Protonation of key histidine residues has been long implicated in the acid-mediated cellular action of the diphtheria toxin translocation (T-) domain, responsible for the delivery of the catalytic domain into the cell. The function of the T-domain is to translocate the catalytic domain across the lipid bilayer in response to the acidification of the endosome. Remarkably, such a complex task is performed by this small 180-residue protein without the help of any additional translocation machinery. Formation of the membrane-competent W+-state occurs in solution upon acidification of the environment to pH below 6 and is accompanied by structural destabilization and partial unfolding of the T-domain.

In order to further analyze the putative pH-dependent structuring of the TH2-TH3 region, we crystallized a full-length form of diphtheria toxin (DT) harboring the H223Q/H257Q mutations. Notably, two crystal forms were obtained from crystallization solutions at pH 5.5 and 4.5. The first crystal form (DT-DM-A) was isomorphous with the aforementioned WT structures, whereas the other form (DT-DM-B) belonged to another crystal form. Not surprisingly, the mutant structures also form domain-swapped dimers and are similar to the WT structures. Interestingly, the TH2 helices in the mutant structures are well ordered in a similar manner as observed for the WT pH 7.0 structure and could be modeled on the electron density maps. Interestingly, the Q223/Q257 sidechain conformations are distinctly different from the H223/H257 residues in the WT structures. Moreover, the acid-induced destabilization of the T-domain’s short helix TH2, previously reported for the WT, is no longer observed with the DM. The latter is overall consistent with the spectroscopic evidence presented above in Figure 2 for the lack of efficient conversion of the membrane-competent state in the mutant. The replacement of H223 and H257 with non-titratable Q residues suppresses the ability of the T-domain to form a membrane-competent state and disrupt the bilayer yet has little effect on the protonation of the other four histidines.

>MGADDVVDSSKSFVMENFSSYHGTKPGYVDSIQKGIQKPKSGTQGNYDDDWEGFYSTDNKYDAAGYSVDNENPLSGKAGGVVKVTYPGLTKVLALKVDNAETIKKELGLSLTEPLMEQVGTEEFIKRFGDGASRVVLSLPFAEGSSSVKYINNWEQAKALSVELEINFETRGKRGQDAMYEYMAQACAGNRVRRSVGSSLSCINLDWDVIRDKTKTKIESLKEQGPIKNKMSESPNKTVSEEKAKQYLEEFHQTALEQPELSELKTVTGTNPVFAGANYAAWAVNVAQVIDSETADNLEKTTAALSILPGIGSVMGIADGAVHHNTEEIVAQSIALSSLMVAQAIPLVGELVDIGFAAYNFVESIINLFQVVHNSYNRPAYSPGHKTQPFLHDGYAVSWNTVEDSIIRTGFQGESGHDIKITAENTPLPIAGVLLPTIPGKLDVNKSKTHISVNGRKIRMRCRAIDGDVTFCRPKSPVYVGNGVHANLHVAFHRSSSEKIHSNEISSDSIGVLGYQKTVDHTKVNSKLSLFFEIKSMA[2x]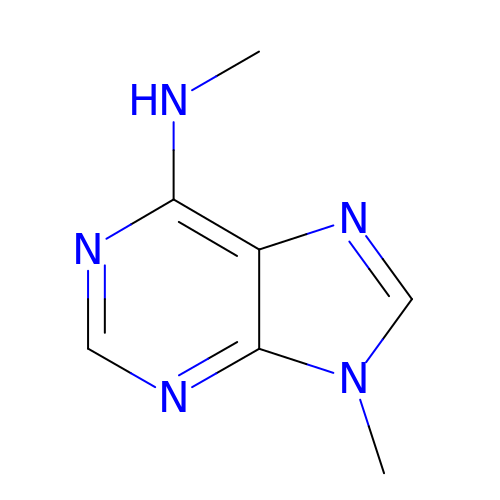~{N},9-dimethylpurin-6-amine | C7 H9 N5 | GRDLXXJSRHDATN-UHFFFAOYSA-N3N-methyl-5N-(4-oxidanylcyclohexyl)-1-[(1S)-1-phenylethyl]pyrazole-3,5-dicarboxamide 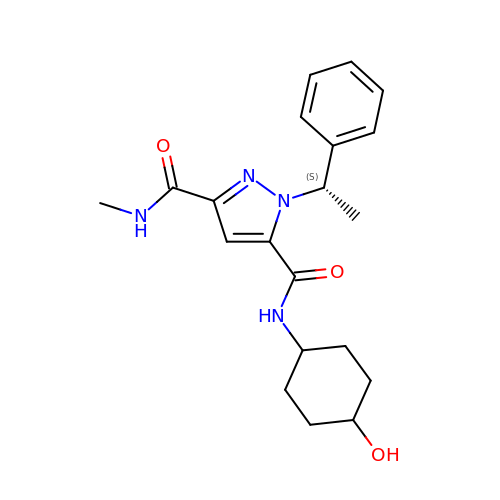| C20 H26 N4 O3 | LEXSRVMWXAFLMV-BPUTZDHNSA-N>MAHHHHHHMEGSVQNKERLWTKRRHAKQLKLEMANQYTDGVVIPTQDIIKVLETLITPGDKVVLEGNNQKQADFLSRSLAQTNPDILHDLHMIMPSVGRSEHLDLFEKGIARKLDFSFAGPQSLRISQLIEDGLLEIGAIHTYIELYSRLVVDLIPN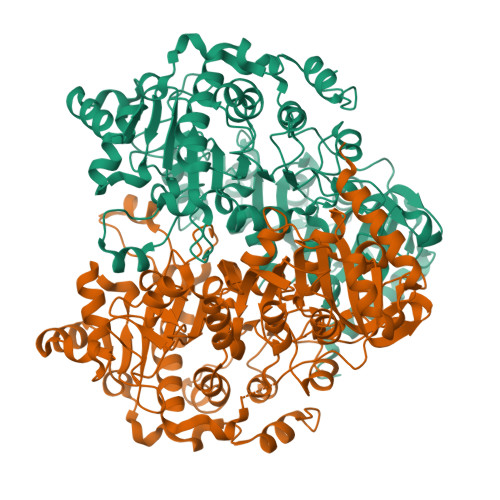VVLSAGFMADRQGNIYTGPSTEDSPALIEPAAFSDGIVIVQVNELVDDVSELPRVDIPASWVDYVVVADQPFYIEPLFTRDPKHIKPVHVLMAMMAIRGIYEKHNVQSLNHGIGFNTAAIELILPTYGESLGLKGKICRNWTLNPHPTLIPAIETGWVESVHCFGTELGMEKYVAARPDVFFTGRDGALRSNRMMCQLAGQYAVDLFIGATLQVDGMGHSSTVTKGRLAGFGGAPNMGHDPRGRRHDTPAWLDMRLQGANETETYLARGKKLVVQMVETFQEGGKPTFVDRLDAIDVAKTAGLPLAPIMIYGDDVTHLLTEEGIAYLYKASSQEERQAMIAAVAGVTSIGLTQDPKTTARLRREGLVVFPEDLGIRRTDATRELLAAKNIADLVTWSDGLYQPPAKFRSW[2x]>MNIVLMGLPGAGKGTQAEKIVAKYGIPHISTGDMFRAAMKEETPLGLEAKSYIDKGELVPDEVTIGIVRERLSKSDCERGFLLDGFPRTVAQAEALEEILEEMGRKLEHVIHIDVRQEELMERLTGRRICSVCGTTYHLVF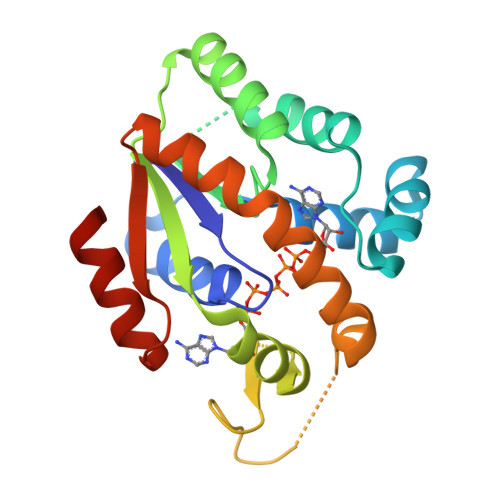NPPKTPGICDKDGGELYQRADDNEETVAKRLEVNMKQMKPLLAFYDSKEVLRNVNGEQDMEKVFKDLRELLQGLAR[4x]> MPKHGKRYRALLEKVDPNKIYTIDEAAH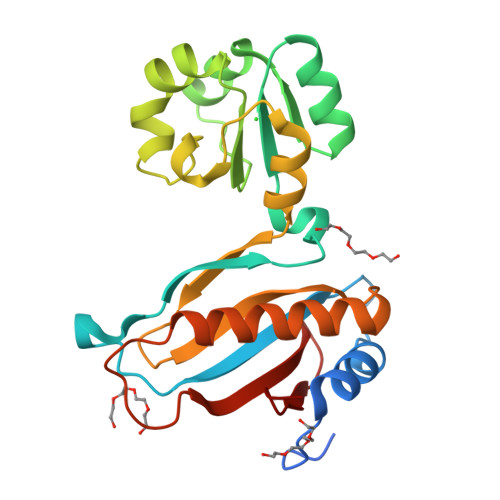LVKELATAKFDETVEVHAKLGIDPRRSDQNVRGTVSLPHGLGKQVRVLAIAKGEKIKEAEEAGADYVGGEEIIQKILDGWMDFDAVVATPDVMGAVGSKLGRILGPRGLLPNPKAGTVGFNIGEIIREIKGRIEFRNDKTGAIHAPVGKASFPPEKLADNIRAFIRALEAHKPEGAKGTFLRSVYVTTTMGPSVRINPHS>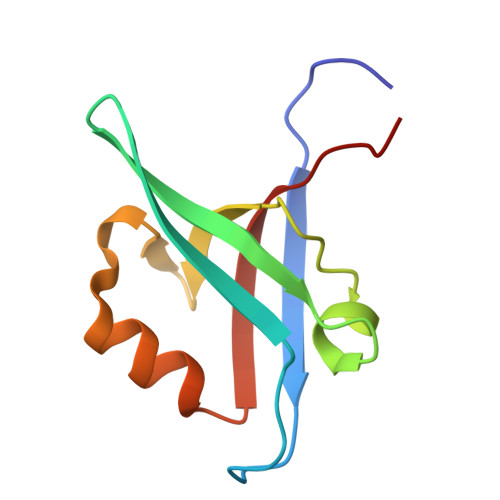 GAMGKVTHSIHIEKSDTAADTYGFSLSSVEEDGIRRLYVNSVKETGLASKKGLKAGDEILEINNRAADALNSSMLKDFLSQPSLGLLVRTYPEL> HNHNHNHNHNHNGGENLYFQGASLTEIEHLVQSVCKSYRETCQLRLEDLLRQRSNIFSREEVTGYQRKSMWEMWERCAHHLTEAIQYVVEFAKRLSGFMELCQNDQIVLLKAGAMEVVLVRMCRAYNADNRTVFFEGKYGGMELFRALGCSELISSIFDFSHSLSALHFSEDEIALYTALVLINAHRPGLQEKRKVEQLQYNLELAFHHHLCKTHRQSILAKLPPKGKLRSLCSQHVERLQIFQHLH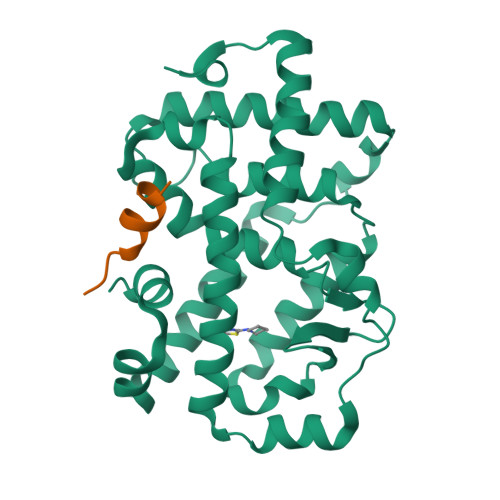PIVVQAAFPPLYKELFSGG;> KHKILHRLLQDS Here, a high-throughput approach to determine room-temperature damage-free structures with excellent sample and time efficiency is demonstrated, allowing complexes to be characterized rapidly and without prohibitive sample requirements. We have applied this approach to crystals of two heme peroxidase enzymes: a multifunctional dehaloperoxidase from the marine annelid Amphitrite ornata (DHP-B; Barrios et al., 2014; Franzen et al., 2012; McCombs, Moreno-Chicano, et al., 2017; McCombs, Smirnova et al., 2017) and a dye-decolourizing peroxidase of industrial relevance from Streptomyces lividans (DtpAa). We also examine the challenging case of detecting nitrite binding to copper nitrite reductase from Achromobacter cycloclastes (AcNiR; Horrell et al., 2017), where the ligand displaces a water molecule bound in the active site. Our results cover several different ligand-binding scenarios, such as coordinate-bond formation to a heme iron (imidazole) or copper (nitrite) and noncoordinate ligand binding in a pocket (DHP ligands), with the latter being highly relevant to the binding of ligands to pharmacologically important proteins such as cytochromes P450.

The overall structure of the enzyme homodimer was highly similar to that of ferric DtpAa crystallized in a condition that did not contain imidazole. c difference maps indicated that an imidazole ligand was coordinated via an N atom to the distal position of the heme iron in one monomer of the DtpAa dimer with full occupancy. The Fe—N (imidazole) bond was 2.2 Å, while imidazole also formed two hydrogen bonds (2.7 and 2.9 Å) to Asp239 [Fig. 1(c)], and the heme pocket also contains several well ordered water molecules. Comparison with the ligand-free ferric DtpAa structure also obtained by SFX revealed that the imidazole displaces the distal water molecule from the heme and induces a number of modest structural rearrangements in the heme pocket. A second imidazole molecule is bound to the protein away from the heme pocket, forming a 2.7 Å bond to Thr351 and interacting via a bridging water with Glu283. In contrast, for monomer A no imidazole ligand was observed in the distal heme pocket and instead a water molecule is bound at a distance of 2.4 Å in a similar manner to that in the ferric DtpAa structure. The imidazole ligand provided a more challenging case owing to its smaller size in comparison to DCP and 5BR and because of the lower symmetry space group (P21) of the DtpAa crystals. For the latter reason, the merging statistics deteriorated more rapidly than for DHP. In a lower symmetry space group (DtpAa; P21), the ability to detect ligand binding in data sets of <2000 images was compromised by a lack of data completeness at higher resolution, although ligand finding was still achieved with 800 images.

>[2x]AGSAVPFHGAHQAGIATPVQDRLHFAAFDVTTEDRAAFVALLKEWTAAARRLTAGHAVGEGAYGGLPEAPPDDTGEALGLKPSRLTLTIGFGPSLFTRFGLADLRPEALADLPKFPGDNLDRARSGGDLCVQACADDPQVAVHAIRNLARIGFGKVVVRWSQLGFGKTSSTTPDKQTPRNLLGFKDGTRNIAGTEKDRLDRFVWAAEKDGTPWMTGGSYLVARRIRMHIETWDRASLQEQEDVFGRDKGEGAPVGKAKERDEPFLKAMKPDAHVRLAHPDSNGGATLLRRGYSFTDGTDGLGRLDAGLFFLAYQRDIRTGFVPVQRNLATDALNEYIQHVGSAVFAVPPGVRDADDWWGSTLF>GSHMDSTTIQQNKDTLSQIVVFPTGNYDKNEANAMVNRLANIDGKYLNALKQNNLKIKLLSGKLTDEKEYAYLKGVVPKGWEGTGKTWDDVPGLGGSTVALRIGFSNKGKGHDAINLELHETAHAIDHIVLNDISKSAQFKQI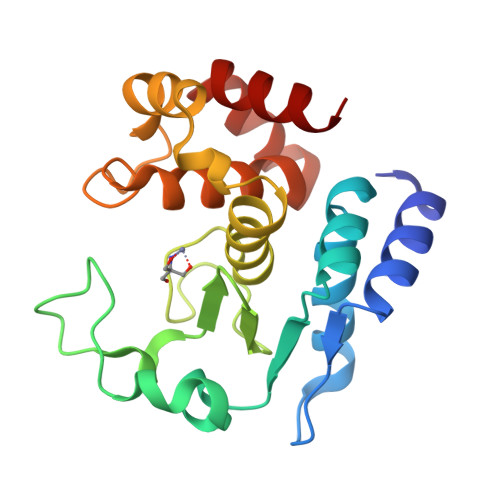FAKEGRSLGNVNYLGVYPKEFFAESFAYYYLNQDTNSKLKSACPQTYSFLQNLAK[2x]>MGSSHHHHHHSSGLEVLFQGPAERISKQSTPFVGAQIFIEPGQTQEQIEQWFKLLAESNMTTCRIRMFGKYMKTPSGTYDFTLFDRAFKLADKYHIKVYATLFPDTEFTDVGGFKFPHSREHQKEVEDYIKNVVSHFSQYKNLAAWVLINEPGTPNLPFNEPFTKERFSDWKKEHNFSEYNEKGYPVLNFEKENFIIDYHNWYLNWLANQVRLYDKQHDLHVNPHNVFKLSGLYDFPTWRTFLNSLGGSAHASWHFGYFPRKAYTVAMSANAELIRSGAGELPWLMTELQGGNNLYSGANPLCPTAEEIIQWLWINFATEAKGGIFWSFNARSTAAEAGEWAMINFKNKSSDRLIAAATIGKFITENVKMMSNIKTLNSGISILYNHESMWVEAAQTRGKLNGNGRSIGAVMCSPLSYFEALSETGLQANFKEIKEFDFSLNDYTD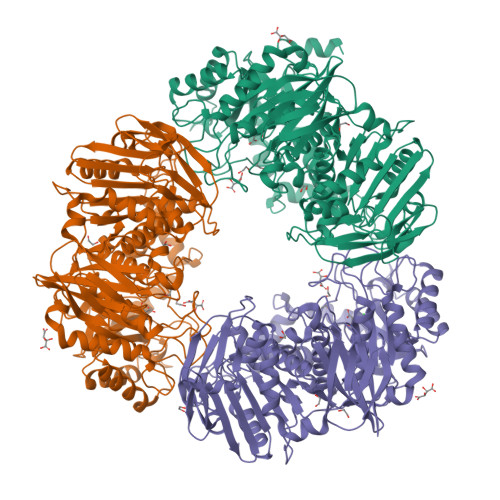QVIILSHQIALDNKVIKQLESFVEKGGTLIADGLTGYYDYQAHSTVVSGFALENLFGSYPIEYKIKENLFSLDFEKDNYKLPAHLWKGTIETSKATPIMDKEGECIACINQYGKGKVFWIPSPIALGARESKDFSELSKLTVSLLPNKILNDNPHFDKHYKDVMMKSFKSNGTMYSLIINKSASVQTVDIVGGKGKAFILFANKNAHSTANKLTISPEETVIIKWKNN[6x]5,6-bis(4-fluorophenyl)-8-oxidanyl-3~{H}-quinazolin-4-one | C20 H12 F2 N2 O2 | 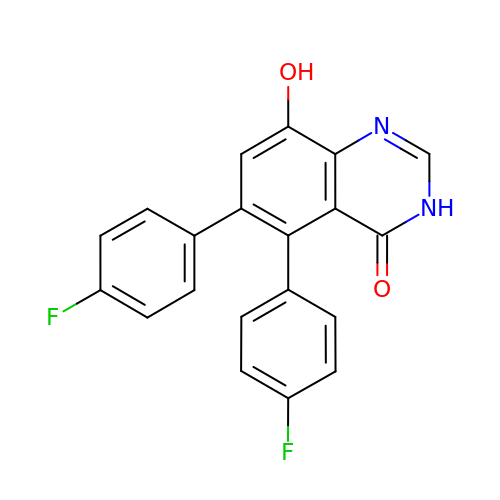XHKWMBTVWDSDBK-UHFFFAOYSA-N>[2x]GAMASTTLETRDELTPQMKEYDRAGRVWVPYLNYFHRPNHRSPVVNTDSRGFRFVVGKDGRTFSEFEREPGERVRALVGGSTVFGVGATGDAATLPSLLSQRGPARWLNFGGRAFSSTQELMLFLF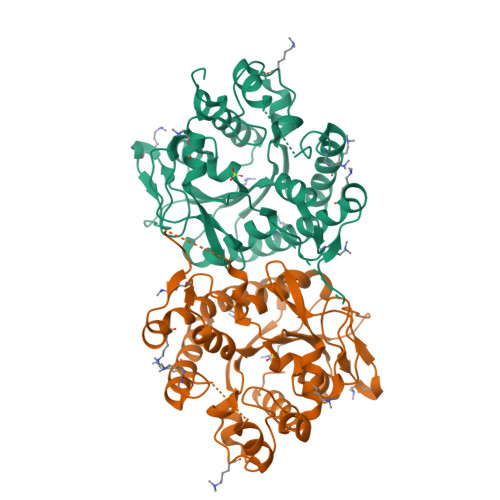HARSLGALEKVTLLSGVNNLLLFYLSRDYAKDYGSFFATEVRRAFAGDAPSPAKSGVIGRLKSIAGGRRAKVEAPEPEIVLPIVDHDAQKTDLLHAIERDLSTWKLLSGALQFELCYVLQPLAGWVRKKPSPEETRLFADLDDQQGEAWRQILREKMDLAQYAWFSKSLADICRTQEIPFLDMNATLSALDLDGRWIFVDRVHLTDEGNEVLTQALVEGGAT>MSLNKKVFIIDKQTVYQEIDNFSASDAWRCAFIGKNWPQEKKEKIADLLFKREFDEKGNPIGMALTNWRVNIGAGSYENREAKEVDNSWNRTECFLSPDGKYDFTKQAGQQWFMKAARERGMNNFLFFTNSAPYFMTRSASTVSTDQDCINLQNDKFDDFARFLVKSAQHFREQGFHVNYISPNNEPNGQWHANSFQEGSFATKADLYRMVEELDKAISEAQIDTKILIPEVGDMKYLFEIDSIAKTPDDIIHSMFYKDGQYSVLKFKNLFNCVAAHDYWSAYPATLLVDIRNRIHKELSANGHNTKFWASEYCILEKNEEITMPASPERSINLGLYVARIIHNDLTLANASAWQWWTAVSLGEDVPIQLLPLEGSNGLSLQYDGEISTTKMLWTTANYSFFVRP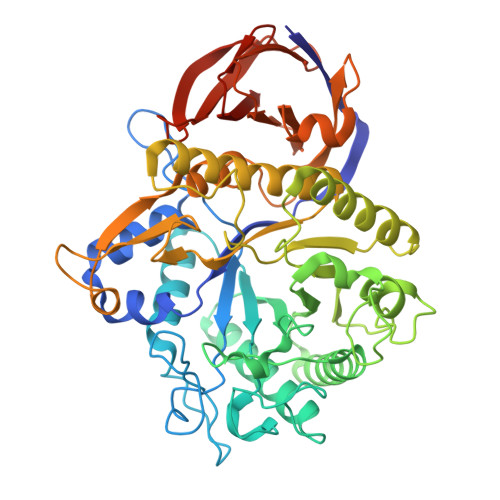GMKRIAIKPTYKISDLEAATSLMISSYTDGKEVVTVAINYSKENQVISLNCDHAQKGKVYLTTIDKNLRYMGEQPLKKLQLPARSVATIVVEDNEGHHHHHH[6x]>[2x]AYTTFSQTKNDQLKEPMFFGQPVNVARYDQQKYDIFEKLIEKQLSFFWRPEEVDVSRDRIDYQALPEHEKHIFISNLKYQTLLDSIQGRSPNVALLPLISIPELETWVETWAFSETIHSRSYTHIIRNIVNDPSVVFDDIVTNEQIQKRAEGISSYYDELIEMTSYWHLLGEGTHTVNGKTVTVSLRELKKKLYLCLMSVNALEAIRFYVSFACSFA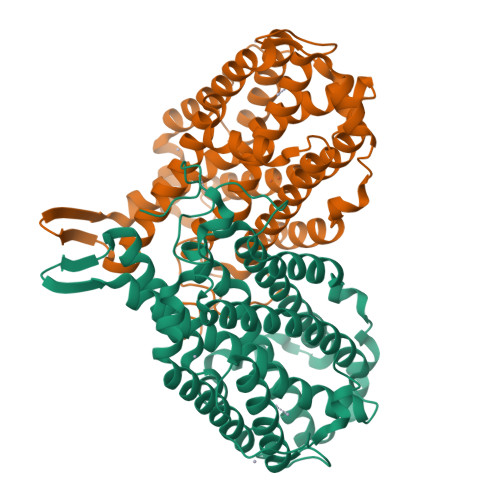FAERELMEGNAKIIRLIARDEALHLTGTQHMLNLLRSGADDPEMAEIAEECKQECYDLFVQAAQQEKDWADYLFRDGSMIGLNKDILCQYVEYITNIRMQAVGLDLPFNTRSNPIPWINTWLVSDNVQVAPQEVEVSSYLVGQIDSEVDTDDLSNFQL>[6x]MSITLRTYIFLDALQPQLATFIGKTARGFLPVPGQASLWVEIAPGIAINRVTDAALKATKVQPAVQVVERAYGLLEVHHFDQGEVLAAGSTILDKLEVREEGRLKPQVMTHQIIRAVEAYQTQIINRNSQGMMILPGESLFILETQPAGYAVLAANEAEKAANVHLVNVTPYGAFGRLYLAGSEAEIDAAAEAAEAAIRSVSGVAQESFRDR;>MDHAPERFDATPPAGEPDRPALGVLELTSIARGITVADAALKRAPSLLLMSRPVSSGKHLLMMRGQVAEVEESMIAAREIAGAGSGALLDELELPYAH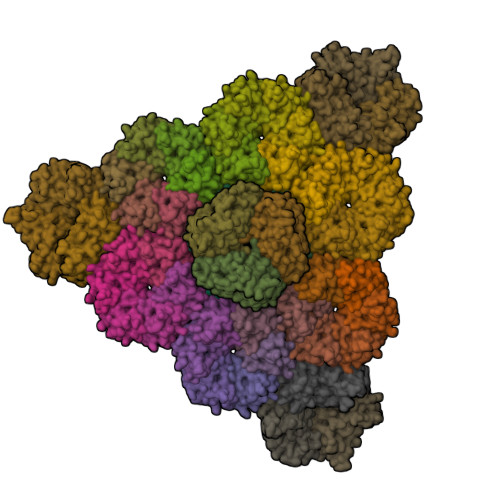EQLWRFLDAPVVADAWEEDTESVIIVETATVCAAIDSADAALKTAPVVLRDMRLAIGIAGKAFFTLTGELADVEAAAEVVRERCGARLLELACIARPVDELRGRLFF[9x];>[36x]MADALGMIEVRGFVGMVEAADAMVKAAKVELIGYEKTGGGYVTAVVRGDVAAVKAATEAGQRAAERVGEVVAVHVIPRPHVNVDAALPLGRTPGMDKSA> GSHMLD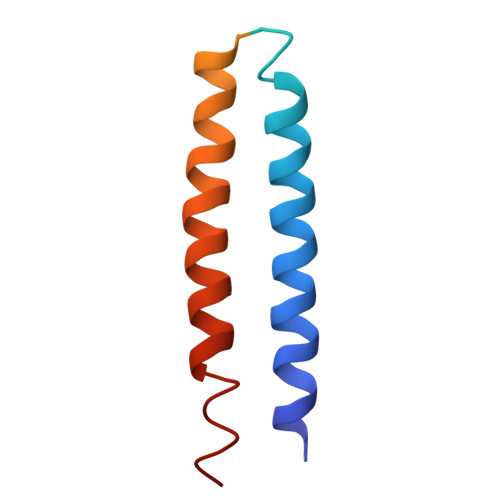RILSIRKSRANRLRESMAKINSQIKEVDGKLDDCEQSIKESIASKQAYCASLVNLDKVSLYKYQIKNNAFDEQKQRLYEKKSSLSKEKRSLLDSQKRTKENLQHVNKSVEKLSFAIKEHYFD> MSVTVKRIIDNTVIVPKLPANEDPVEYPADYFRKSKEIPLYINTTKSLSDLRGYVYQGLKSGNVSIIHVNSYLYGALKDIRGKLDKDWSSFGINIGKAGDTIGIFDLVSLKALDGVLPDGVSDASRTSADDKWLPLYLLGLYRVGRTQMPEYRKKLMDGLTNQCKMINEQFEPLVPEGRDIFDVWGNDSNYTKIVAAVDMFFHMFKKHECASFRYGTIVSRFKDCAALATFGHLCKITGMSTEDVTTWILNREVADEMVQMMLPGQEIDKADSYMPYLIDFGLSSKSPYSSVKNPAFHFWGQLTALLLRSTRARNARQPDDIEYTSLTTAGLLYAYAVGSSADLAQQFCVGDNKYTPDDSTGGLTTNAPPQGRDVVEWLGWFEDQNRKPTPDMMQYAKRAVMSLQGLREKTIGKYAKSEFDK;>[2x]MSSLKKILGLKGKGKKSKKLGIA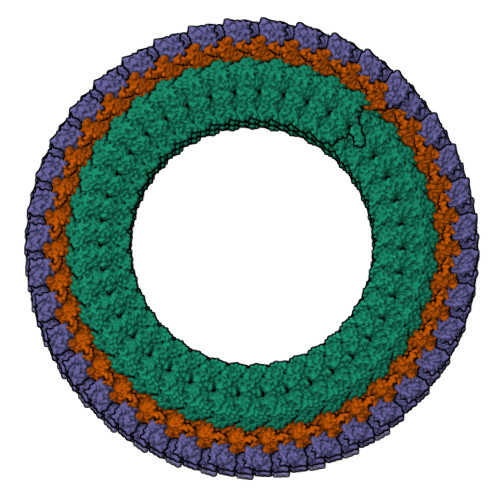PPPYEEDTSMEYAPSAPIDKSYFGVDEMDTYDPNQLRYEKFFFTVKMTVRSNRPFRTYSDVAAAVSHWDHMYIGMAGKRPFYKILAFLGSSNLKATPAVLADQGQPEYHAHCEGRAYLPHRMGKTPPMLNVPEHFRRPFNIGLYKGTIELTMTIYDDESLEAAPMIWDHFNSSKFSDFREKALMFGLIVEKKASGAWVLDSISHFK> AEQKTLHIYNWSDYIAPDTVANFEKETGIKVVYDVFDSNEVLEGKLMAGSTGFDLVVPSAYFLERQLTAGVFQPLDKSKLPEWKNLDPELLKLVAKHDPDNKFAMPYMWATTGIGYNVDKVKAVLGENAPVDSWDLILKPENLEKLKSCGVSFLDDPEEVFATVLNYLGKDPNSTKADDYTGPATDLLLKLRPNIRYFHSSQYINDLANGDICVAIGWAGDVWQASNRAKEAKNGVNVSFSIPKEGAMAFFDVFAMPADAKNKDEAYQFLNYLLRPDVVAHISDHVFYANANKAATPLVSAEVRENPGIYPPADVRAKLFTLKVQDPKIDRVRTRAWTKVKSGKLEHHHHHH

Here, we present a fluorescence-based, genetically encoded AGM biosensor, consisting of an AGM binding-domain derived from the putrescine periplasmic binding-protein (PBP) PotF from *E. coli* fused to a super-folder circularly permuted GFP (sfcpGFP). In the sensor the large conformational change of the PBP upon ligand binding is transmitted to the fluorescent protein by altering the chromophore environment and thus triggering a change in signal. We chose PotF due to its promiscuous binding of biogenic amines characterized in prior studies. Previously, we identified AGM as a natural ligand (K_D_ = 0.22 µM) for the periplasmic binding-protein PotF.

We confirmed the effect of these mutations on AGM specificity by measuring binding affinities with ITC for the PotF receptor module without the fluorescence protein: PotF-S87Y-A182D displayed an affinity of 0.3 µM for AGM and no apparent K_D_ for the other tested ligands PUT, SPD, and CDV ([Fig figs3]). To examine and understand the binding of AGM further, we solved the crystal structure of PotF-S87Y-A182D in complex with AGM and compared it to the wild-type PotF structure. Interestingly, the two lobes of PotF are slightly more open in the S87Y-A182D construct ([Fig fig2]). We analyzed the relative orientation of the lobes in this structure and found 10.9° wider opening and 7.1° wider twisting angles compared to wild type like closure. Still, most AGM interacting residues in the binding pocket do not differ ([Fig fig1] & [Fig fig2]). Since the lobes are slightly further apart, distances between interacting residues and important binding pocket water molecules can change. These distances are compensated by the bulkier ligand AGM but are most probably detrimental for high affinity binding of slim ligands like PUT and SPD. The main structural changes occur in the distal site of the pocket (S87Y & A182D, [Fig fig1] & [Fig fig2]) where the guanidino group of AGM is located. It appears that this larger and bulkier group withstands the mutational changes and maintains high affinity while the smaller primary amine groups of other ligands lose most of their affinity.>MMIVIKTAIPDVLILEPKVFGDERGFFFESYNQQTFEELIGRKVTFVQDNHSKSKKNVLRGLHFQRGENAQGKLVRCAVGEVFDVAVDIRKESPTFGQWVGVNLSAENKRQLWIPEGFAHGFVTLSEYAEFLYKATNYYSPSSEGSILWNDEAIGIEWPFSQLPELSAKDAAAPLLDQALLT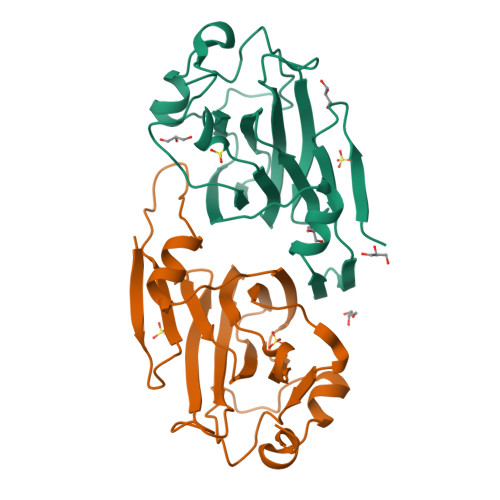E[2x]>[2x]SKILVFGHQNPDSDAIGSSMAYAYLKRQLGVDAQAVALGNPNEETAFVLDYFGIQAPPVVKSAQAEGAKQVILTDHNEFQQSIADIREVEVVEVVDHHRVANFETANPLYMRLEPVGSASSIVYRLYKENGVAIPKEIAGVMLSGLISDTLLLKSPTTHASDPAVAEDLAKIAGVDLQEYGLAMLKAGTNLASKTAAQLVDIDAKTFELNGSQVRVAQ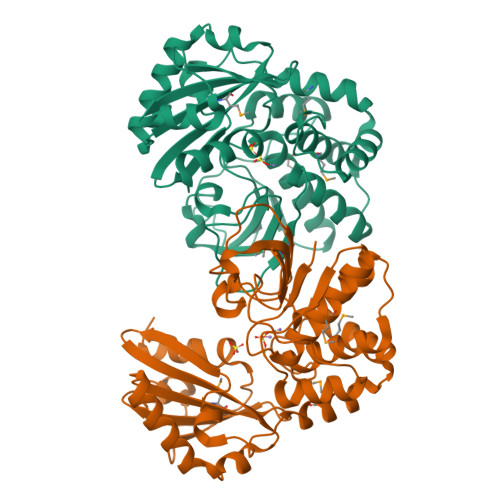VNTVDINEVLERQNEIEEAIKASQAANGYSDFVLMITDILNSNSEILALGNNTDKVEAAFNFTLKNNHAFLAGAVSRKKQVVPQLTESFNG>MITKLMIDEKYAKELDKAEIDHHKPTAGAMLGHVLSNLFIENIRLTQAGIYAKSPVKCEYLREIAQREVEYFFKISDLLLDENEIVPSTTEEFLKYHKFITEDPKAKYWTDEDLLESFIVDFQAQNMFITRAIKLANKEEKF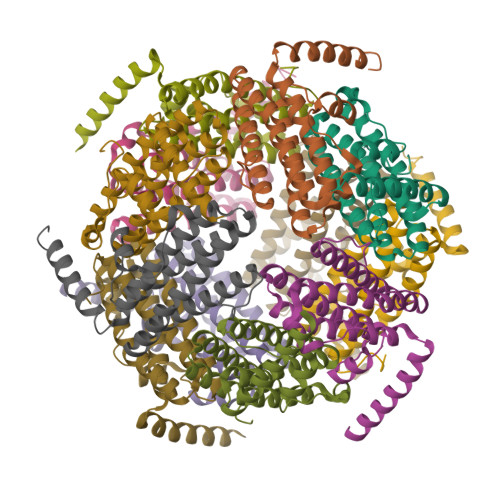ALAAGVVELYGYNLQVIRNLAGDLGKSVADFHDEDEDNDN[12x]>MKSLQALFGGTFDPVHYGHLKPVETLANLIGLTRVTIIPNNVPPHRPQPEANSVQRKHMLELAIADKPLFTLDERELKRNAPSYTAQTLKEWRQEQGPDVPLAFIIGQDSLLTFPTWYEYETILDNAHLIVCRRPGYPLEMAQPQYQQWLEDHLTHNPEDLHLQ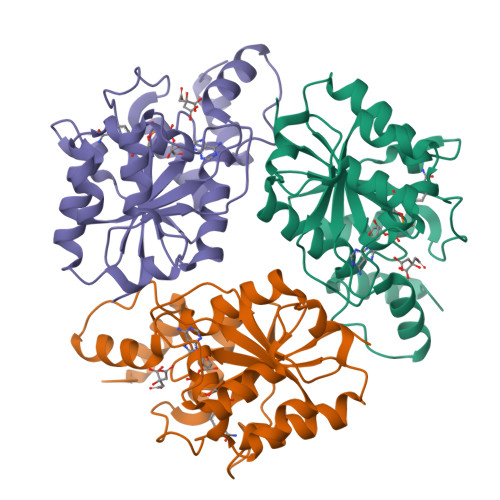PAGKIYLAETPWFNISATIIRERLQNGESCEDLLPEPVLTYINQQGLYR[3x]> MKRVMFHAKIHRATVTQA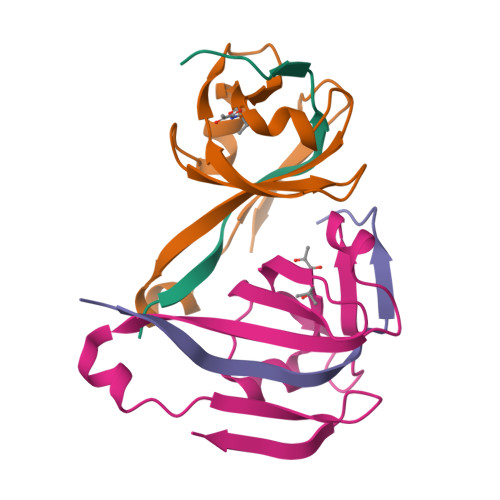DLHYVG;> XVTVDQDLLDAAGILPFEQVDIYDITNGARLTTYALPGERGSGVIGINGAAAHLVKPGDLVILVAYGVFDEEEARNLKPTVVLVDERNRILEVRKG2-ethyl-2-(hydroxymethyl)propane-1,3-diol | C6 H14 O3 | 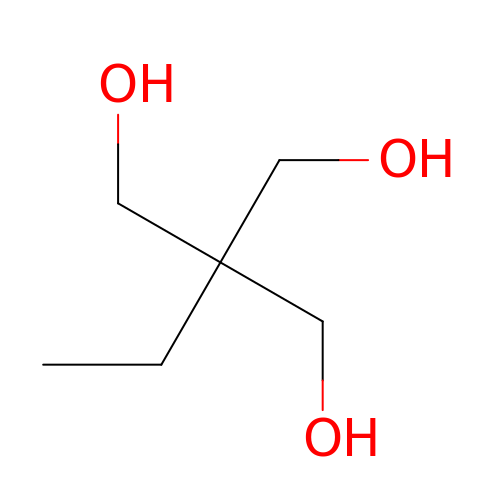ZJCCRDAZUWHFQH-UHFFFAOYSA-N> GFRGVEEKKSLEILLKDDRLDTEKLCTFSQRFPLPSMYRALVWKVLLGILPPHHESHAKVMMYR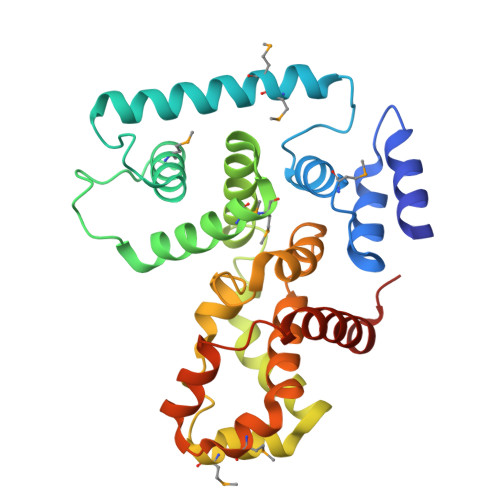KEQYLDVLHALKVVRFVSDATPQAEVYLRMYQLESGKLPRSPSFPLEPDDEVFLAIAKAMEEMVEDSVDCYWITRRFVNQLNTKYRDSLPQLPKAFEQYLNLEDGRLLTHLRMCSAAPKLPYDLWFKRCFAGCLPESSLQRVWDKVVSGSCKILVFVAVEILLTFKIKVMALNSAEKITKFLENIPQDSSDAIVSKAIDLWHKHCGTPVHSS Toll-like Receptor 3 (TLR3) is a pattern recognition receptor that initiates antiviral immune responses upon binding double-stranded RNA (dsRNA). The extracellular domain is responsible for ligand recognition and contains multiple leucine-rich repeats (LRRs) that form a horseshoe-like structure. Here, we use computational protein design to create novel miniproteins that bind to human TLR3 with nanomolar affinities. Cryo-EM structures of two minibinders in complex with TLR3 reveal that they bind the target as designed, although one partially unfolds due to steric competition with a nearby N-linked glycan.

Following a strategy previously established for structural characterization of TLR4/MD-2 complexes, we co-expressed the TLR3 ectodomain and each minibinder in HEK293F cells and co-purified the complexes using affinity chromatography followed by SEC. This improved occupancy, and after optimizing grid preparation and data collection to overcome a clear preferred orientation, we determined cryo-EM structures of minibinders 7.7 and 8.6 in complex with TLR3, each at 2.9 Å resolution. Minibinders 7.7 and 8.6 interacted with the concave surface of TLR3 in slightly different manners, with α1 and α2 of minibinder 7.7 binding to LRR15-LRRCT and α2 and α3 of minibinder 8.6 binding to LRR13-LRRCT. Unlike minibinder 8.6, for which clear density was observed for all three α-helices, we could build only α1 and α2 of minibinder 7.7 into well-defined density. Interestingly, density corresponding to α3 of minibinder 7.7 could be observed extending from α2 at a low threshold (0.08σ). Given the proximity of the minibinder to the glycan at N413, we conclude that a steric clash between the glycan and minibinder 7.7 makes α3 protrude out from the complex. This conclusion is supported by our SSM data for minibinder 7—obtained in complex with TLR3—which showed that mutations in the hydrophobic core were more tolerated than would be expected for a well-folded protein. For minibinder 8.6, the α2 and α3 helices were well-aligned (Cα RMSD: 1.6 Å), but α1 was slightly displaced from its predicted position (Cα RMSD: 2.7 Å). The altered conformation of minibinder 7.7 α3 described above may result in exposure of hydrophobic residues in the protein core to solvent (e.g., L11 and L30). The interactions between minibinder 7.7 and TLR3 were mainly mediated through electrostatic interactions. Residues E9, Y25, K28, and K32 of minibinder 7.7 were crucial for forming electrostatic interactions with TLR3. Due to a nearby glycan, the third helix of minibinder 7.7 was disordered when bound to TLR3, a phenomenon that has not been documented before in designed minibinders to the best of our knowledge.

> KCTVSHEVADCSHLKLTQVPDDLPTNITVLNLTHNQLRRLPAANFTRYSQLTSLDVGFNTISKLEPELCQKLPMLKVLNLQHNELSQLSDKTFAFCTNLTELHLMSNSIQKIKNNPFVKQKNLITLDLSHNGLSSTKLGTQVQLENLQELLLSNNKIQALKSEELDIFANSSLKKLELSSNQIKEFSPGCFHAIGRLFGLFLNNVQLGPSLTEKLCLELANTSIRNLSLSNSQLSTTSNTTFLGLKWTNLTMLDLSYNNLNVVGNDSFAWLPQLEYFFLEYNNIQHLFSHSLHGLFNVRYLNLKRSFTKQSISLASLPKIDDFSFQWLKCLEHLNMEDNDIPGIKSNMFTGLINLKYLSLSNSFTSLRTLTNETFVSLAHSPLHILNLTKNKISKIESDAFSWLGHLEVLDLGLNEIGQELTGQEWRGLENIFEIYLSYNKYLQLTRNSFALVPSLQRLMLRRVALKNVDSSPSPFQPLRNLTILDLSNNNIANINDDMLEGLEKLEILDLQHNNLARLWKHANPGGPIYFLKGLSHLHILNLESNGFDEIPVEVFKDLFELKIIDLGLNNLNTLPASVFNNQVSLKSLNLQKNLITSVEKKVFGPAFRNLTELDMRFNPFDCTCESIAWFVNWINETHTNIPELSSHYLCNTPPHYHGFPVRLFDTSSCKDSA;> SAMEYYVKELLRTAEYAREAGDPEYVRKALEKAELVARILHNEELKEEIREVEEEL S-BENZOYLTHIAMINE O-MONOPHOSPHATE 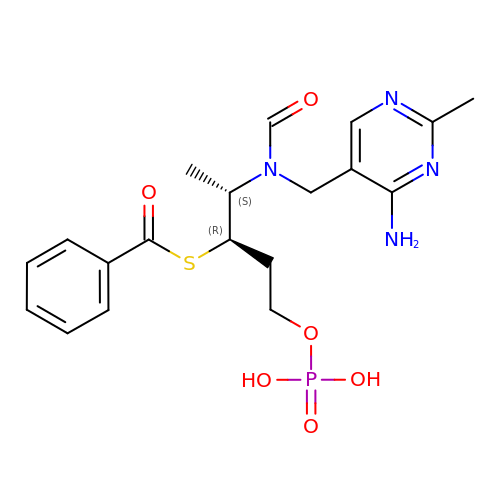| C19 H25 N4 O6 P S | ZVFWYYRSRJTRQB-SUMWQHHRSA-N> DEPGVATGNGQPVTGNWLAGASQGDGVPIPSQIADQLRGKEFKSWRDFREQFWMAVSKDPSALENL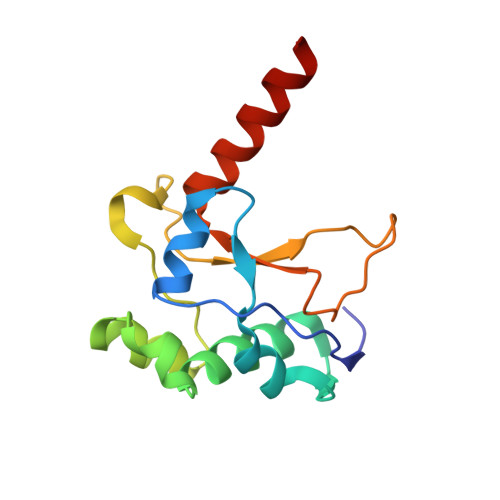SPSNRYFVSQGLAPYAVPEEHLGSKEKFEIHHVVPLESGGALYNIDNLVIVTPKRHSEIHKELKLKRKEK>[2x]GPMAWASSFDAFFKNFKRESKIISEYDITLIMTYIEENKLQKAVSVIEKVLRDIESAPLHIAVTGETGAG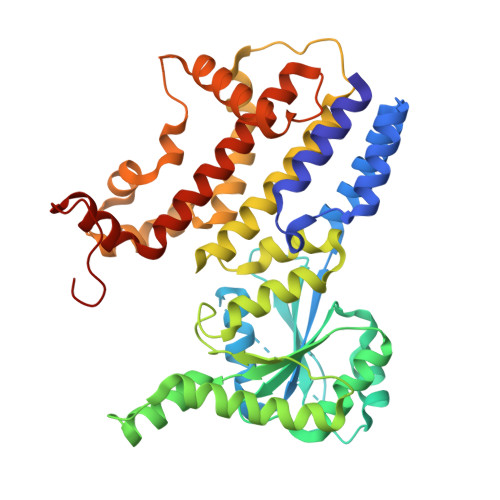KSTFINTLRGVGHEEKGAAPTGAIETDMKRTPYPHPKLPNVTIWDLPGIGTTNFTPQNYLTEMKFGEYDFFIIISATRFKENDAQLAKAIAQMGMNFYFVRTKIDSDLDNEQKFKPKSFNKEEVLKNIKDYCSNHLQESLDSEPPVFLVSNVDISKYDFPKLETKLLQDLPAHKRHVFSLSLQSLTEATINYKRDSLKQKVFLEAMKAGALATIPLGGMISDILENLDETFNLYRSYFGLDDASLENIAQDLNMSVDDFKVHLRFPHLFAEHNDESLEDKLFKYIKHISSVTGGPVAAVTYYRMAYYLQNLFLDTAANDAIALLNSKALFEKKVGPYISEPPEYWEA>MMASAATELDVDG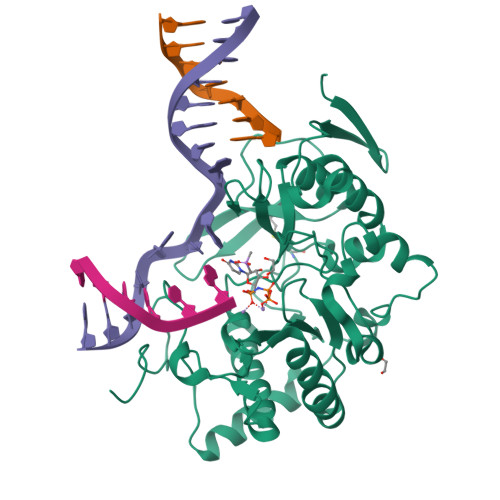VKVRFTNPDKVYFPKLGKNGTKGKLVEYYLSVASGPMLALLRDRPVHLQRFPDGIEGEEIYQKRVPQKHPDYLETCVVTFPSGRTADALKITHPSSIIWAAQMGTVTLHPWQVRCPDTEHPDELRVDLDPQPGTGFKEARTVACDVLKPLLDELGLVGYPKTSGGRGVHVFLRIKPQWDFIEVRRAGIALAREVERRAPDAVTTSWWKEERGERLFIDYNQNARDRTFASAYSVRKTPIATVSMPLSWDELRNADPDDYTMNTVPDLLAGRDDPWADIDSVQQSLGPLLDLVAADEERGLGDLPYPPNYPKMPGEPPRVQPSKKVAEHWDEQGNRKQ[2x]>DPEFGAGGPWEMRERLGTGGFGNVCLYQHRELDLKIAIKSCRLELSTKNRERWCHEIQIMKKLNHANVVKACDVPEELNILIHDVPLLAMEYCSGGDLRKLLNKPENCCGLKESQILSLLSDIGSGIRYLHENKIIHRDLKPENIVLQDVGGKIIHKIIDLGYAKDVDQGELCTEFVGTLQYLAPELFENKPYTATVDYWSFGTMVFECIAGYRPFLHHLQPFTWHEKIKKKDPKCIFACEEMSGEVRFSSHLPQPNSLCSLIVEPMENWLQLMLNWDPQQRGGPVDLTLKQPRCFVLMDHILNLKIVHILNMTSAKIISFLLPPDESLHSLQSRIERETGINTGSQELLSETGISLDPRKPASQCVLDGVRGCDSYMVYLFDKSKTVYEGPFASRSLSDCVNYIVQD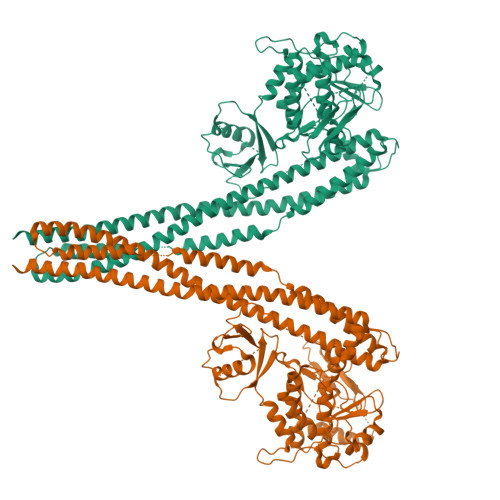SKIQLPIIQLRKVWAEAVHYVSGLKEDYSRLFQGQRAAMLSLLRYNANLTKMKNTLISASQQLKAKLEFFHKSIQLDLERYSEQMTYGISSEKMLKAWKEMEEKAIHYAEVGVIGYLEDQIMSLHAEIMELQKSPYGRRQGDLMESLEQRAIDLYKQLKHRPSDHSYSDSTEMVKIIVHTVQSQDRVLKELFGHLSKLLGCKQKIIDLLPKVEVALSNIKEADNTVMFMQGKRQKEIWHLLKIACTQ[2x]>MNFPQLSKEVAEDEAEVILHTSQGDIRIKLFPKLAPLAVENFLTH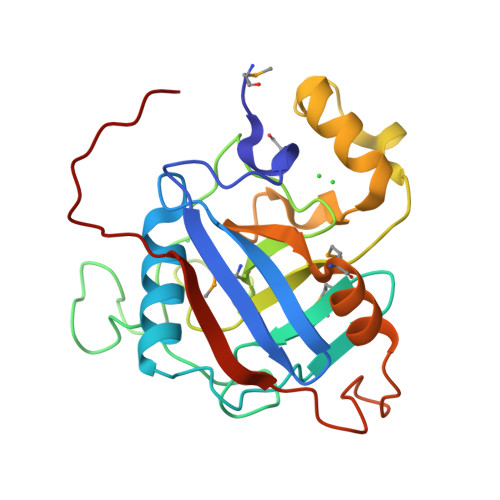AKEGYYNGITFHRVIDGFMVQTGDPKGDGTGGQSIWHDKDKTKDKGTGFKNEITPYLYNIRGALAMANTGQPNTNGSQFFINQNSTDTSSKLPTSKYPQKIIEAYKEGGNPSLDGKHPVFGQVIGGMDVVDKIAKAEKDEKDKPTTAITIDSIEVVKDYDFKSENLYFQ[10x]>GSHMGSASEQRVTLTNADKVLYPATGTTKSDIFDYYAGVAEVMLGHIAGRPATRKRWPNGVDQPAFFEKQLALSAPPWLSRATVAHRSGTTTYPIIDSATGLAWIAQQAALEVHVPQWRFVAEPGSGELNPGPATRLVFDLDPGEGVMMAQLAEVARAVRDLLADIGLVTFPVTSGSKGLHLYTPLDEPVSSRGATVLAKRVAQRLEQAMPALVTSTMTKSLRAGKVFVDWSQNSGSKTTIAPYSLRGRTHPTVAAPRTWAELDDPALRQLSYDEVLTRIARDGDLLERLDADAPVADRLTRY[4x]

Nonhomologous end-joining (NHEJ) is one of the major DNA double-strand break (DSB) repair pathways. Mycobacterial LigD comprises three distinct enzymatic domains: DNA ligase, phosphoesterase (PE), and a polymerase (PolDom). PE and PolDom of LigD remodel incompatible DNA termini for ligation. Archaeo-prokaryotic (AP) NHEJ polymerases (PolDom or LigD Pol) are members of the archaeo-eukaryotic primase (AEP) superfamily (Aravind and Koonin, 2001; Weller and Doherty, 2001; Iyer et al., 2005; Bartlett et al., 2013).

To understand the molecular basis for the proposed in trans templated polymerization extensions, PolDom was crystallized in complex with dsDNA containing a self-complementary 3′ overhang. The DNA substrate consisted of a template (T) strand (ten bases) annealed to a recessed downstream (D) strand (5 bases), resulting in a 5 bp 3′ overhang on the T strand. The complex consists of two PolDom monomers (residues 10–293), each bound to a DNA “end” forming two PolDom-DNA binary complexes. The binary complexes are brought together by a continuous molecular cradle, formed by the polymerases, that promotes synapsis between the discontinuous DNA termini. The 3′-overhanging template strands are further stabilized by a region of microhomology, formed by four Watson-Crick base pairs (G7-C10). PolDom interacts with the recessed 5′ phosphate of the downstream strand, noted previously (Brissett et al., 2007, 2011) and splays the templating strand at the ds/ss junction by ∼119°. The templating strand from one binary complex appears to terminate in the active site of the opposing PolDom monomer. This configuration effectively makes the outgoing “templating” strand from one binary complex an incoming “primer” strand for the other monomer and exemplifies the term in trans for this complex. For this transition to occur, the highly conserved loop 2 (residues 213–224), particularly residues Met215, Lys217, and Arg220 make direct contacts with the incoming 3′ strand and channel it toward the neighboring polymerase active site. Lys235 and Asp227 directly contact the primer terminus, and Gln230, Ser229, and Asp137 also form part of this hydroxyl recognition pocket.>HHHHHHHHMPHMEDNGSEKEQLFLQHIQNLPQERLDAIRGHPELVLKEIDEFTYPDGSGVRMCIGDVKGGFIVGKIRERKPKIMVELGGYLGYSAILFGNEISKIPGGRYYSLEVNEDYAKIAYELVKLAGLDEIVTIMIGKACDSLVELQQKLLHKDLGFQALDMVFIDHWKDLYVPDLRVIESLNMIAPGTLLVADNIITPGAPEYHKY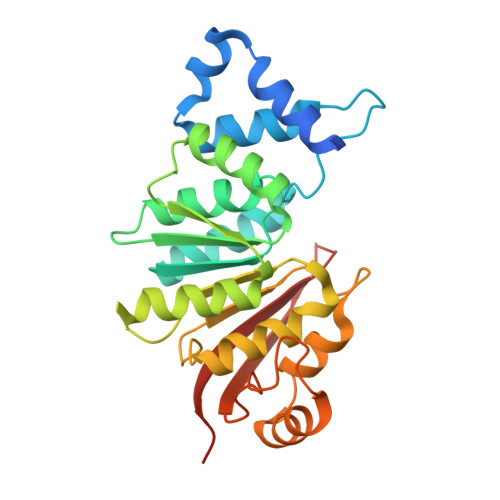VNMSPEERRGYQAKVRNVNGFDFIGRWDLIYKTETKEFEGVIRNKHRKDAVDVTECVGYAKKD[2x]> MDLRRRPPKPPVTNNNNSNGSFRSYQPRTSDDDHRRRATTIAPPPKASDALPLPLYLTNAVFFTLFFSVAYYLLHRWRDKIRYNTPLHVVTITELGAIIALIASFIYLLGFFGIDFVQSFISRASGDAWDLADTIDDDDHRLVTCSPPTPIVSVAKLPNPEPIVTESLPEEDEEIVKSVIDGVIPSYSLESRLGDCKRAASIRREALQRVTGRSIEGLPLDGFDYESILGQCCEMPVGYIQIPVGIAGPLLLDGYEYSVPMATTEGCLVASTNRGCKAMFISGGATSTVLKDGMTRAPVVRFASARRASELKFFLENPENFDTLAVVFNRSSRFARLQSVKCTIAGKNAYVRFCCSTGDAMGMNMVSKGVQNVLEYLTDDFPDMDVIGISGNFCSDKKPAAVNWIEGRGKSVVCEAVIRGEIVNKVLKTSVAALVELNMLKNLAGSAVAGSLGGFNAHASNIVSAVFIATGQDPAQNVESSQCITMMEAINDGKDIHISVTMPSIEVGTVGGGTQLASQSACLNLLGVKGASTESPGMNARRLATIVAGAVLAGELSLMSAIAAGQLVRSHMKYNRSSRDISGATTTTTTTT

HMGR (3-hydroxy-3-methylglutaryl-coenzyme A reductase) is the rate limiting enzyme of the eukaryotic mevalonate pathway successfully targeted by statins to treat hypercholesterolemia in humans. As HMGR inhibitors have been shown to be herbicidal, HMGR could represent a mode of action target for the development of herbicides. Here, we present the crystal structure of a HMGR from Arabidopsis thaliana (AtHMG1) which exhibits a wider active site than previously determined structures from different species. By contrast, the conserved extracellular domain of AtHMG1 shares ~54% sequence identity with HsHMGCR and strictly conserved catalytic residues.

To develop plant-specific statins and mitigate off-target effects, we solved the crystal structure of the core domain of apo AtHMG1 and in complex with pitavastatin to resolutions of 1.9 and 2.1 Å, respectively, in space groupI 41 2 2. Closer inspection of the statin-binding pocket revealed two substitutions in AtHMG1 with respect to HsHMGCR located at the hydrophobic CoA binding region of the active site pocket, specifically, Ile562/Leu857 and Ile389/Val683 in AtHMG1/HsHMGCR respectively. Furthermore, a plant conserved Val to Pro (Pro236/Val530 A. thaliana/human) substitution at the start of the Lβ1-strand is the likely cause of conformational flexibility and lack of electron density in the Nα4-Lβ1 loop adjacent to the active site-delineating Lβ2-Lα1 loop. This flexibility results in the loss of a type II β-turn found within the HsHMGCR Lβ2-Lα1 loop that is stabilised by hydrogen bonding between a conserved Glu (Glu234/Glu528 AtHMG1/HsHMGCR) and a Cys backbone amine (Cys267/Cys561 AtHMG1/HsHMGCR). Importantly, the arrangement of the AtHMG1 Lβ2-Lα1 loop results in Glu265 being unable to form a hydrogen bond with the O5-hydroxyl group of the HMG moiety of statins or the equivalent thioester oxygen of HMG-CoA, as it is shifted 2.5 Å away, creating a wider pocket. The differences in the architecture of AtHMG1 that allowed for species selectivity largely arise from an unusual orientation of the Lβ2-Lα1 loop that is likely the result of increased flexibility in the neighbouring Nα4-Lβ1 loop. The atypical orientation of the Lβ2-Lα1 loop in AtHMG1 disrupts the hydrogen bonding network formed between the catalytic residues Glu265/Lys397/Asn461/Asp473 (HsHMGCR Glu559/Lys691/Asn755/Asp767), thereby retaining only those hydrogen bonds that stabilise the catalytic Lys via the adjacent Asn and Asp residues. Glu265 is not in a favourable position to hydrogen bond to either the substrate thioester oxygen or the adjacent Asp473, which based on HsHMGCR in silico simulations (HsHMGCR Glu559 and Asp767) might be expected to hydrogen bond and stabilise the mevaldyl-CoA intermediate.>GSGEEVSEEGFQIPATITERYKVGRTIGDGNFAVVKECVERSTAREYALKIIKKSKCRGKEHMIQNEVSILRRVKHPNIVLLIEEMDVPTELYLVMELVKGGDLFDAITSTNKYTERDASGMLYNLASAIKYLHSLNIVHRDIKPENLLVYEHQDGSKSLKLGDFGLATIVDGPLYTVCGTPTYVAPEIIAETGYGLKVDIWAAGVITYILLCGFPPFRGSGDDQEVLFDQILMGQVDFPSPYWDNVSDSAKELITMMLLVDVDQRFSAVQVLEHPWVNDDGLPENEHQLSVAGKIKKHFNTGPKPNSTAAGV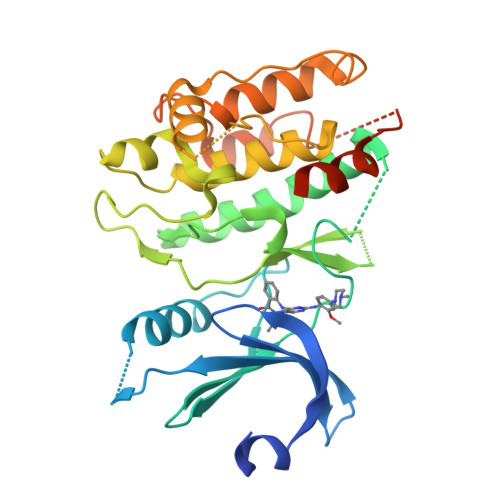SVIA[2x]>[2x]SNARFSDVHGCDEAKEELQELVEFLRNPEKFSNLGGKLPKGVLLVGPPGTGKTLLARAVAGEAGVPFFYMSGSEFDEIYVGVGAKRVRELF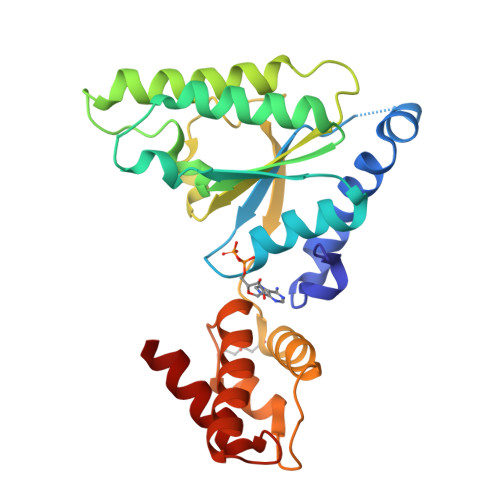NAAKAKAPSIVFIDELDAIGGRRNSRDATYVRQTLNQLLTEMDGFAQNSGVIILGATNFPESLDKALTRPGRFDRHVHVSLPDVRGRIAILKHHAKKIKIGSDVNIAAIAARTSGLSGAELENIVNQAAVHASKEKAKAVMQAHFEWAKDKVIMG SA lipase (SAL, also known as glycerol ester hydrolase), a triacylglycerol esterase, shows strong cytopathic activity in host cells. SAL, an ester bond-hydrolyzing enzyme, is secreted in prepolypeptide form containing 690 amino acid residues and is processed into its mature form containing 394 amino acid residues. Its active site is composed of a typical catalytic triad including Ser116, Asp 307, and His349 residues, similar to other serine hydrolases. The SAL crystal structure exhibited a typical α/β-hydrolase fold comprising a central twisted β-sheet flanked by α-helices on both sides.

The crystal structure of native SAL was determined using MR techniques. The Staphylococcus hyicus lipase (SHL) chain A of 2hih16, which shares 47.7% identity with that of SAL, was used as a search model using the CCP4 Phaser program. Final values of the general R-factor and free R-factor up to a resolution of 2.08 Å were 21.3% and 23.5%, respectively. The dimeric refined model comprised 764 amino acids with 76 solvent molecules with 2 zinc and 2 calcium ions and 12 fatty acid fragments of various lengths. The native SAL structure was observed as an open form. In the native SAL crystal structure, dimer interactions were typically hydrophobic. Remarkably, fatty acid branches were located between the dimer interface, which should stabilize the dimeric form of SAL. In the native SAL crystal, three fatty acids were observed near the active site, whereas only one fragment was bound to S116A mutant. SAL specifically hydrolyzes triacylglycerol, and these three fatty acids may reflect a triacylglycerol position for hydrolysis. The other four long fatty acids were also found bound far from active sites on chains A and B of the SAL structure, particularly at the lid of α-helix 7 and helix 8. This also blocked the lid domain from moving forward to the active site, thereby maintaining the lid in its open form.

>[2x]MNHKVHHHHHHMKANQVQPLNKYPVVFVHGFLGLVGDNAPALYPNYWGGNKFKVIEELRKQGYNVHQASVSAFGSNYDRAVQLYYYIKGGRVDYGAAHAAKYGHERYGKTYKGIMPNWEPGKKVHLVGHSMGGQTIRLMEEFLRNGNKEEIAYHQAHGGEISPLFTGGHNNMVASITTLATPHNGSQAADKFGNTEAVRKIMFALNRFMGNKYSNIDLGLTQWGFKQLPNESYIDYIKRVSKSKIWTSDDNAAYDLTLDGSAKLNNMTSMNPNITYTTYTGVSSHTGPLGYENPDLGTFFLMDTTSRIIGHDAREEWRKNDGVVPVISSLHPSNQPFVNVTNNEPATRRGIWQVKPILQGWDHVDFIGVDFLDFKRKGSELANFYIGIINDLLSVEATEGKGTQLKAS> ENLKPPENIDVYIIDDNYTLKWSSHGESMGSVTFSAEYRTKDEAKWLKVPECQHTTTTKCEFSLLDTNVYIKTQFRVRAEEGNSTSSWNEVDPFIPFYTAHMSPPEVRLEAEDKAILVHISPPGQDGNMWALEKPSFSYTIRIWQKSSSDKKTINSTYYVEKIPELLPETTYCLEVKAIHPSLKKHSNYSTVQCIST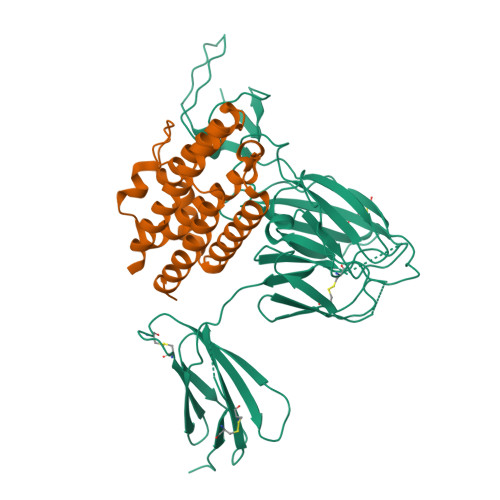TVANKMPVPGNLQVDAQGKSYVLKWDYIASADVLFRAQWLPGYSKSSSGSRSDKWKPIPTCANVQTTHCVFSQDTVYTGTFFLHVQASEGNHTSFWSEEKFIDSQKHILPPPPVITVTAMSDTLLVYVNCQDSTCDGLNYEIIFWENTSNTKISMEKDGPEFTLKNLQPLTVYCVQARVLFRALLNKTSNFSEKLCEKTRPGSFST;> INYKQLQLQERTNIRKCQELLEQLNGKINLTYRADFKIPMEMTEKMQKSYTAFAIQEMLQNVFLVFRNNFSSTGWNETIVVRLLDELHQQTVFLKTVLEEKQEERLTWEMSSTALHLKSYYWRVQRYLKLMKYNSYAWMVVRAEIFRNFLIIRRLTRNFQN>MNPFHELEPGPEVPEVVYALIEIPKGSRNKYELDKKTGLLKLDRVLYSPFFYPVDYGIIPQTWYDDGDPFDIMVIMREPVYPLTIIEARPIGIMKMEDSGDKDWKVLAVPVEDPYFNDWKDI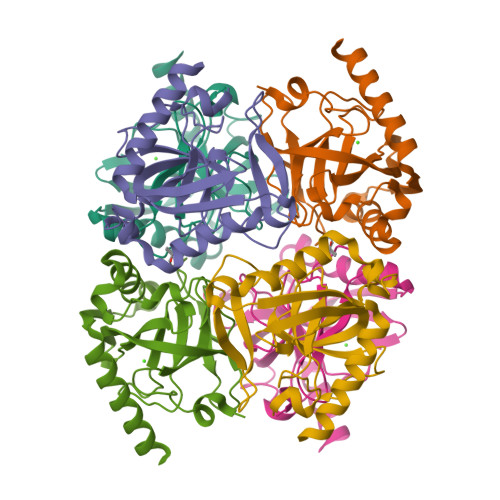SDVPKAFLDEIAHFFQRYKELQGKTTKIEGWGNAEEAKREILRAIEMYKEKFGKEE[6x]> SNASFDETSKRNEGRVKNIVYLDFDGTITGAHGKEVISSPLCEALSTKAT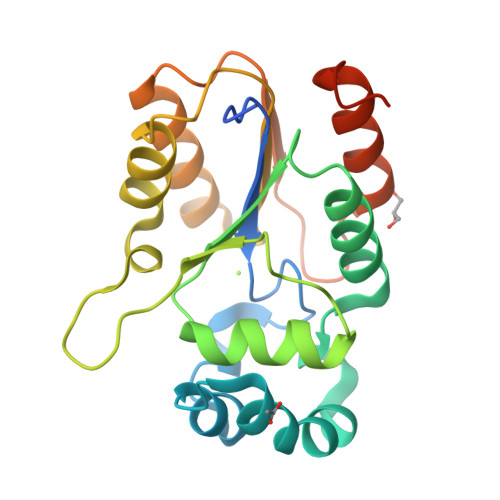FDERMRYKNEYDASDNKIKITENAKNFLQDVNKLHPQVKIVIISRNHENYIKALLEFENIDHRNIIIYPRGVGNTIGPGEDKYKAVVSHEEKPECLPGFRLICDDDEVDGEEMCNGLIHTGRSQLVKFHNEKPGQFKWGEYFKEILTNCDIAVKEYLNGKIGSRFH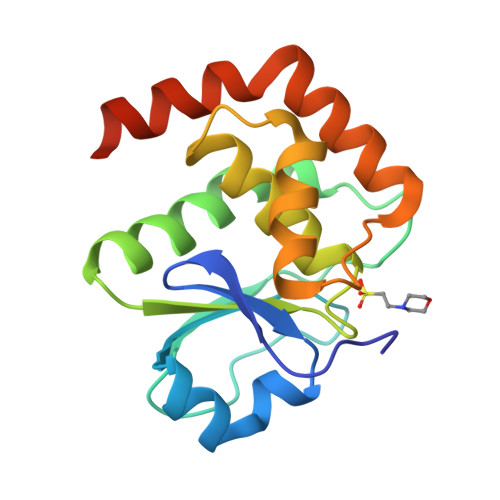> GPMGNGMNKILPGLYIGNFKDARDAEQLSKNKVTHILSVHDSARPMLEGVKYLCIPAADSPSQNLTRHFKESIKFIHECRLRGESCLVHCLAGVSRSVTLVIAYIMTVTDFGWEDALHTVRAGRSCANPNVGFQRQLQEFEKHEVHQYRQWLKEEYGESPLQDAE4-[(5-phenyl-1~{H}-imidazol-2-yl)methylamino]-2-(pyridin-3-ylmethoxy)benzenecarboximidamide | C23 H22 N6 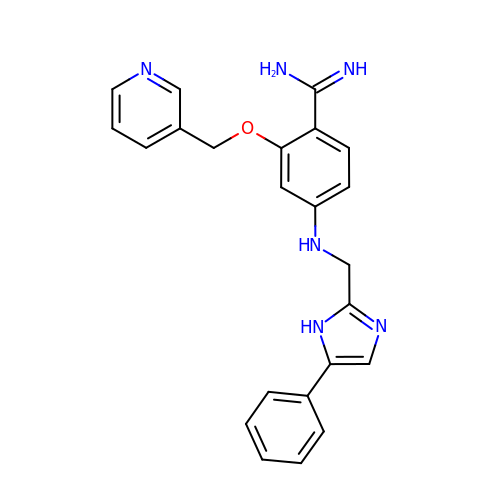O | ZDLCAMFQMDNCSU-UHFFFAOYSA-N> SPKALEEAPWPPPEGAFVGFVLSRKEPMWADLLALAAARGGRVHRAPEPYKALRDLKEARGLLAKDLSVLALREGLGLPPGDDPMLLAYLLDPSNTTPEGVARRYGGEWTEEAGERAALSERLFANLWGR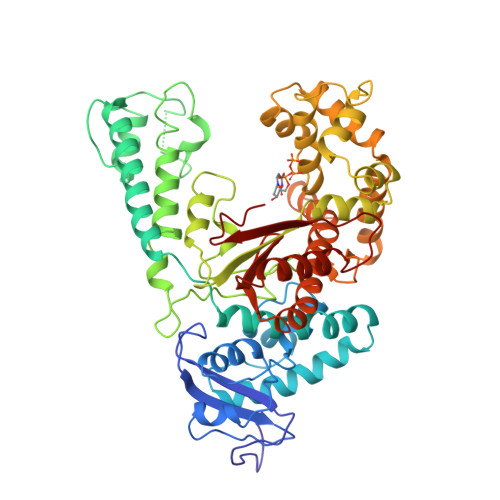LEGEERLLWLYREVERPLSAVLAHMEATGVRLDVAYLRALSLEVAEEIARLEAEVFRLAGHPFNLNSRDQLERVLFDELGLPAIGKTEKTGKRSTSAAVLEALREAHPIVEKILQYRELTKLKSTYIDPLPDLIHPRTGRLHTRFNQTATATGRLSSSDPNLQNIPVRTPLGQRIRRAFIAEEGWLLVALDYSQIELRVLAHLSGDENLIRVFQEGRDIHTETASWMFGVPREAVDPLMRRAAKTINFGVLYGMSAHRLSQELAIPYEEAQAFIERYFQSFPKVRAWIEKTLEEGRRRGYVETLFGRRRYVPDLEARVKSVREAAERMAFNMPVQGTAADLMKLAMVKLFPRLEEMGARMLLQVHDELVLEAPKERAEAVARLAKEVMEGVYPLAVPLEVEVGIGEDWLSAKE> MDFFNLNNNNNNNNTTTTTTTTNNNNTNNNNTNNNNNPANNTNNNNSTGHSSNTNNNTNNNNTNTGASGVDDFQNFFDPKPFDQNLDSNNNNSNSNNNDNNNSNTVASSTNFTSPTAVVNNAAPANVTGGKAANFIQNQSPQFNSPYDSNNSNTNLNSLSPQAILAKNSIIDSSNLPLQAQQQLYGGNNNNNSTGIANDNVITPHFITNVQSISQNSSSSTPNTNSNSTPNANQQFLPFNNSASNNGNLTSNQLISNYAASNSMDRSSSASNEFVPNTSDNNNNSNNHNMRNNSNNKTSNNNNVTAVPAATPANTNNSTSNANTVFSERAAMFAALQQKQQQRFQALQQQQQQQQNQQQQNQQPQQQQQQQQNPKFLQSQRQQQQRSILQSLNPALQEKISTELNNKQYELFMKSLIENCKKRNMPLQSIPEIGNRKINLFYLYMLVQKFGGADQVTRTQQWSMVAQRLQISDYQQLESIYFRILLPYERHMISQEGIKETQAKRIFLQQFLQELLKKVQQQQQAAALANANNNINSASSAPTPAAPGASVPATAAPGTEAGIVPVSANTPKSLNSNININVNNNNIGQQQVKKPRKQRVKKKTKKELELERKEREDFQKRQQKLLEDQQRQQKLLLETKLRQQYEIELKKLPKVYKRSIVRNYKPLINRLKHYNGYDINYISKIGEKIDSNKPIFLFAPELGAINLHALSMSLQSKNLGEINTALNTLLVTSADSNLKISLVKYPELLDSLAILGMNLLSNLSQNVVPYHRNTSDYYYEDAGSNQYYVTQHDKMVDKIFEKVNNNATLTPNDSNDEKVTILVDSLTGNQLPTPTPTEMEPDLDTECFISMQSTSPAVKQWDLLPEPIRFLPNQFPLKIHRTPYLTSLKKIKDEIDDPFTKINTRGAEDPKVLINDQLSTISMILRNISFSDNNSRIMSRNFYLKRFISDLLWLVLIHPENFTCNRKILNFKKDLVIVLSNISHLLEIASSIDCLLILILVISFGQPKLNPMASSSSFGSESLTFNEFQLQWGKYQTFGVDILAKLFSLEKPNLNYFKSILLNKNTGNNLYDRNSNNNHKDKKLLRRLLNLYNDNNKNNNNRHNLLNDVVSFLFSAIPLQQVLSQSADPSLLIDQFSPVISQSLTSILVIVQKILPLSNEVFEISENNSDSNSNNNGNKDSSFNFNKNLPFVWLSSEENIGSGLLKLSEIILNINNSTSKN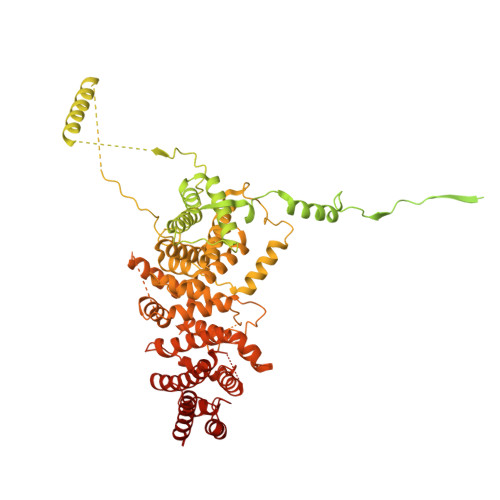TLLQQQNYSKVLLPSINISCVQLIKCLVEKSICFENCLNNDPEILKKIASIPNLFPTDLEIFQLFTNPSVDIQIINQYQLLYNLKNDILTNLE> MAAAAAGAGSGPWAAQEKQFPPALLSFFIYNPRFGPREGQEENKILFYHPNEVEKNEKIRNVGLCEAIVQFTRTFSPSKPAKSLHTQKNRQFFNEPEENFWMVMVVRNPIIEKQSKDGKPVIEYQEEELLDKVYSSVLRQCYSMYKLFNGTFLKAMEDGGVKLLKERLEKFFHRYLQTLHLQSCDLLDIFGGISFFPLDKMTYLKIQSFINRMEESLNIVKYTAFLYNDQLIWSGLEQDDMRILYKYLTTSLFPRHIEPELAGRDSPIRAEMPGNLQHYGRFLTGPLNLNDPDAKCRFPKIFVNTDDTYEELHLIVYKAMSAAVCFMIDASVHPTLDFCRRLDSIVGPQLTVLASDICE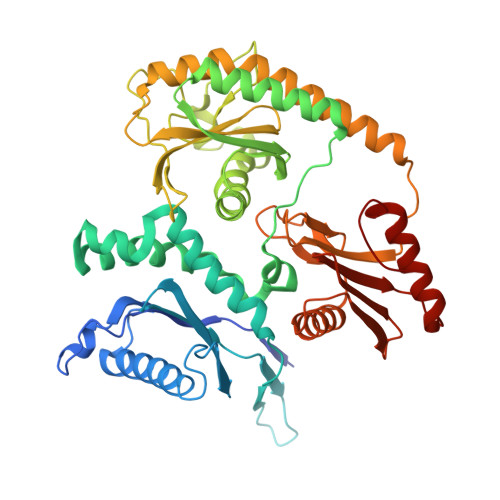QFNINKRMSGSEKEPQFKFIYFNHMNLAEKSTVHMRKTPSVSLTSVHPDLMKILGDINSDFTRVDEDEEIIVKAMSDYWVVGKKSDRRELYVILNQKNANLIEVNEEVKKLCATQFNNIFFLD1-methyl-2-oxo-4-[4-(thiophen-2-ylcarbonyl)piperazin-1-yl]-1,2-dihydroquinoline-3-carbonitrile 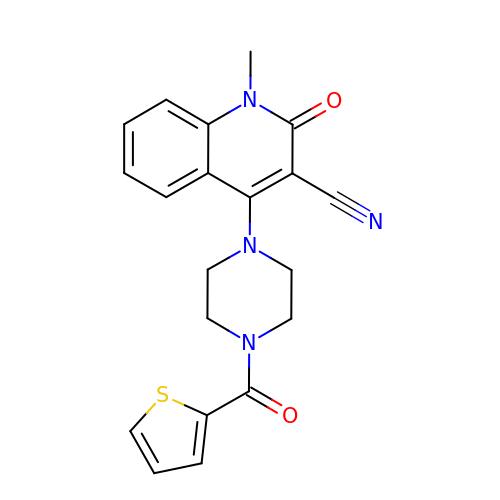| C20 H18 N4 O2 S | GGGJOEPOPVIHEK-UHFFFAOYSA-N> MGSSHHHHHHSSGLVPRGSMSTSWSDRLQNAADMPANMDKHALKKYRREAYHRVFVNRSLAMEKIKCFGFNMDYTLAVYKSPEYESLGFELTVERLVSIGYPQELLSFAYDSTFPTRGLVFDTLYGNLLKVDAYGNLLVCAHGFNFIRGPETREQYPNKFIQRDDTERFYILNTLFNLPETYLLACLVDFFTNCPRYTSCETGFKDGDLFMSYRSMFQDVRDAVDWVHYKGSLKEKTVENLEKYVVKDGKLPLLLSRMKEVGKVFLATNSDYKYTDKIMTYLFDFPHGPKPGSSHRPWQSYFDLILVDARKPLFFGEGTVLRQVDTKTGKLKIGTYTGPLQHGIVYSGGSSDTICDLLGAKGKDILYIGDHIFGDILKSKKRQGWRTFLVIPELAQELHVWTDKSSLFEELQSL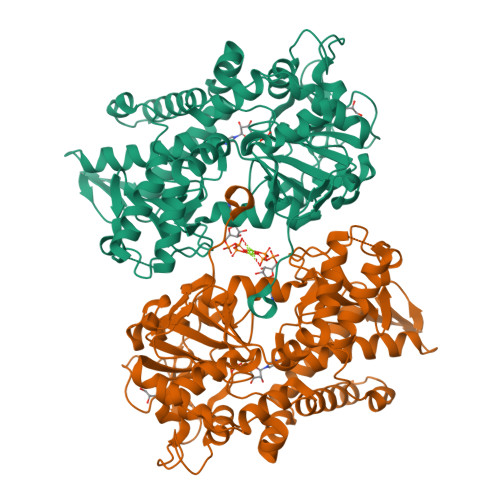DIFLAELYKHLDSSSNERPDISSIQRRIKKVTHDMDMCYGMMGSLFRSGSRQTLFASQVMRYADLYAASFINLLYYPFSYLFRAAHVLMPHESTVEHTHVDINEMESPLATRNRTSVDFKDTDYKRHQLTRSISEIKPPNL>MRVIVFFDLPVITPENRHNYSVFRKYLIKSGFIMQQKSVYSKLVLNLTNRDSIVKSIEKNKPPEGLVEVLTVTEKQYAKMEIIIGESKTEYLNTDERLVVL[2x];> IELSG

Spacer acquisition step in CRISPR-Cas system involves the recognition and subsequent integration of protospacer by the Cas1-Cas2 complex in CRISPR-Cas systems. During the spacer acquisition step, the heterohexameric complex of four Cas1 and two Cas2 proteins preferentially insert a protospacer at the first CRISPR repeat region following the leader sequence. Here we report an anti-CRISPR protein, AcrVA5, and reveal the mechanisms by which it strongly inhibits protospacer integration. AcrVA5 exhibits low binding affinity towards Cas2 and acetylates Cas2 at Lys55 on the binding interface of the Cas2 and AcrVA5 N-terminal peptide complex to inhibit the Cas2-mediated endonuclease activity.

Hence, the Cas2-peptide (1MKIELSGGYICYSIE16) complex was chosen for structural determination. The initial model was further refined by Phenix/refine and rebuilt using Coot, with the final Rfactor and Rfree values of 19.51% and 23.21%, respectively. The complex structure contained one Cas2 dimmer and one AcrVA5 peptide per asymmetric unit, with crystallographic statistics listed in Table 1. The crystal structure of Cas2 reveals a compact dimer structure (protomer A & B) in which each chain is composed of three α-helices and five β-strands (α1: residues 14–29, α2: residues 47–59, α3: residues 74–78, β1: residues 1–8, β2: residues 33–36, β3: residues 39–44, β4: residues 66–73 and β5: residues 81–84). In our structure, the interaction between the AcrVA5-peptide and Cas2 is facilitated by a series of interactions: a hydrogen bond between Lys59 of Cas2 and Ile3 of AcrVA5, as well as non-bond contacts between Lys55 of Cas2 and Leu5 of AcrVA5, Gln58 of Cas2 and Leu5 of AcrVA5, and Lys59 of Cas2 and Ile3 of AcrVA5. The buried surface area of the complex of Cas2 and the AcrVA5 peptide is 434.56 Å2 per molecule, thereby suggesting that this complex could be physiologically relevant. Structure superimposition between two protomers of Cas2 reveals a high similarity in the overall structure with a ferredoxin-like fold with an r.m.s.d of 2.03 Å (overall 88 residues), except for the significant structural conformation variation in the C-terminus. The structural heterogeneity observed in the C-terminus was most likely caused by the interaction between Cas2 and the peptide of AcrVA5. Although the β6–β7 region in the structure of Cas2 is unresolved, the binding of AcrVA5 in the α2 helix of Cas2 causes steric hindrance with the neighboring protospacer. Consistent with the MS results, the K55A mutant rendered Cas2 insensitive to inhibition by AcrVA5 in degradation dsDNA substrates, which shows that Lys55 is a structural determinant dictating Cas2 inhibition by AcrVA5.> KPGKATG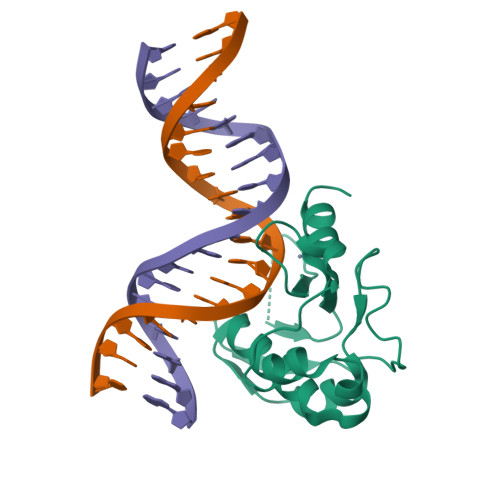KGKPVNNKWLNNAGKDLGSPVPDRIANKLRDKEFKSFDDFRKKFWEEVSKDPELSKQFSRNNNDRMKVGKAPKTRTQDVSGKRTSFELHQEKPISQNGGVYDMDNISVVTPKRHIDIHRGK Complex I couples the transfer of two electrons from NADH to ubiquinone (Q) with the translocation of four protons across the membrane. The L-shaped complex is structured into a peripheral arm that protrudes into the aqueous milieu and catalyzes electron transfer with one FMN and 8–10 iron–sulfur ([Fe–S]) clusters, and a membrane arm embedded in the lipid bilayer that mediates proton translocation. We have determined structures of the electron-input module of complex I from the hyperthermophilic bacterium Aquifex aeolicus, encompassing subunits NuoE and NuoF that contain the FMN cofactor, the [4Fe–4S] cluster N3, and the [2Fe–2S] cluster N1a, respectively, both in the air-oxidized and dithionite-reduced states at resolutions up to 1.8 Å. Here, we show that the redox state of N1a regulates NADH oxidation in complex I by inducing a conformational change close to the NADH-binding site.

We therefore sought to lock the peptide bond in place by exchanging a nearby residue, G129E, with serine and aspartate, respectively. The longer side chains were intended to occupy the position of the bound water molecule that has to make way for the flipping peptide bond according to our structures. Structures of the oxidized G129SE and G129DE variants were refined to 2.4 and 1.9 Å resolution, respectively. Overall, there were no significant changes from the original NuoEF, with the notable exception of the peptide bond of E95F that pointed away from FMN in the oxidized state of both variants, as was the case only in the reduced structures of the original protein. No electron density for ordered water was observed between position 129E and the fixed peptide bond in the variant as determined with NuoEF. The 3.5 Å distance between Oγ of S129E and the carbonyl oxygen of E95F is longer than the 3.2 Å from the carboxylate oxygen of D129E to this position. Thus, while both mutations fixed the position of the peptide bond, the Gly/Asp exchange seemed to exert a much stronger effect than the Gly/Ser mutation.

>[2x]MFKTEFEFPEELKTKLQEHINYFPKKRQAILLCLHEIQNYYGYIPPESLKPLADMLELPLNHVEGVVAFYDMFDREDKAKYRIRVCVSIVCHLMGTNKLLKALENILGIKPGEVTPDGKFKIVPVQCLSACSEAPVFMVNDDEYKFESEVQLNEILSRYT;>MRSYPAIPRIYAETTLNMLLKRAKKPRVHSIDEYLKDGGYQALEKALNMSPEEIIDWVDKSTLRGRGGAGFPTGKKWKFAVQNPGPRYFICNADESEPGTFKDRIIIERDPHLLIEGIIISSYAIGANEAYIYIRGEYPAGYYILRDAIEEAKKKGFLGKNILGSGFDLEIYVARGAGAYICGEETALIESLEGKRGHPRLKPPYPVQKGLWGKPTVVNNVETIANVPFIISMGWEEYRYIGPSDYAGPKLFPVSGKVKKPGVYELPMNTTLREVIFKYAGGTLGNKKVKAVFSGALDCFSSEELDIPMDYSPLGFGGTGTVIVLTEEDDIVEAALKIAEFYEHETCGQCTPCRVGCYEQANLLEKIYKGEATEQDWEGFDFVNRNIQPTSICGLGAVAGRLIRQTLEKFPEEWEKYRKKSASLPLAGHHHHHH[2x]> GAGCAGACTTGA;> CGAGACTCA;> TCATCG;> TCTGAGTCAGTCTGC

In this work, we exhaustively probe the ability of all 36 immobile HJ sequences to form DNA crystals in two different designed systems. Three separate self-assembling DNA crystal systems are described in this report: the “4 × 5” and “4 × 6” designs (collectively referred to as the 4 × N systems), and a third construct with a “scrambled” sequence variant of the 4 × 6 lattices. Self-assembly was mediated by three constituent oligonucleotides: (S1) containing four sequence repeats of either 5 or 6 bases; (S2) composed of 21 bases containing complementary regions to both (S1); and (S3) which forms the second junction crossover. The HJ serves as the fundamental component at the core of each unit, and the ultimate assembly of the full lattice is facilitated by the complementary 2-base sticky ends that tail each duplex.

In parallel, we employed the previously reported J1 4 × 6 system (3.05 Å), with P32 symmetry. Seventeen of the 36 junctions successfully crystallized, a 47% success rate. Unlike the 4 × 5 motif, nearly all of the 4 × 6 junction sequences had a strong preference for crystallization in buffers containing ≥2.0 M salts (e.g., LiCl, Li2SO4, KCl, and NaCl), with the majority preferring slightly basic pH conditions in cacodylic acid. Because the 4 × 6 system yielded R3 symmetry in 5 of 17 junctions, we considered whether the downstream sequences adjacent to the junction could play a role in crystallization efficiency, junction angle, and symmetry preference, or if the HJ alone was the singular determinant. In these scenarios, R3 preferred low concentrations of divalent ions and organic solvents, and P32 required high salt with drastically different lattices. The average cell constants for the P32 crystals were a = b = 68.29 Å c = 55.68 Å. The c-axis, in particular, was ~5 Å shorter, and had a much larger degree of variability (σ = 1.97), than those that crystallized using the 4 × 5 motif. The broad range of the short axis spanned from 52.77 to 60.36 Å, and we posit that the flexible axis lengths could be responsible for rendering a larger number of junctions fatal than the 4 × 5 system. The average junction angles of 54.60° (σ = 1.44) and 58.37° (σ = 2.3) for the P32 and R3 symmetries, respectively, along with their preference for salts or organic solvents, were likely the major contributing factors that yielded the divergent lattices. However, in the majority of the crystal structures reported here, the cacodylate anion indeed fits best into the electron density map of our X-ray structures, due to the presence of sodium cacodylate in the crystallization solution.> LAGVKKDIEKLYEAVPQLSNVFKIEDKIGEGTFSSVYLATAQLQVGPEEKIALKHLIPTSHPIRIAAELQCLTVAGGQDNVMGVKYCFRKNDHVVIAMPYLEHESFLDILNSLSFQEVREYMLNLFKALKRIHQFGIVHRDVKPSNFLYNRRLKKYALVDFGLAQGTHDTKIELLKFVQSEAQQERCSQNKPASLTCDCYATDKVCSICLSRRQQVAPRAGTPGFRAPEVLTKCPNQTTAIDMWSAGVIFLSLLSGRYPFYKASDDLTALAQIMTIRGSRETIQAAKTFGKSILCS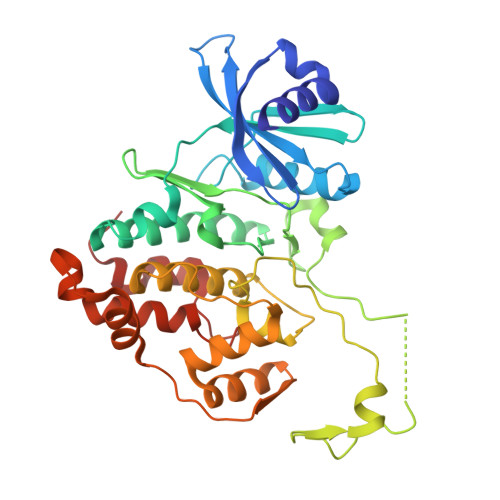KEVPAQDLRKLCERLRGAGAGGWNEVPDEAYDLLDKLLDLNPASRITAEEALLHPFFKDMSL>MSQPITRENFDEWMIPVYAPAPFIPVRGEGSRLWDQQGKEYIDFAGGIAVNALGHAHPELREALNEQASKFWHTGNGYTNEPVLRLAKKLIDATFADRVFFCNSGAEANEAALKLARKFAHDRYGSHKSGIVAFKNAFHGRTLFTVSAGGQPAYSQDFAPLPADIRHAAYNDINSASALIDDSTCAVIVEPIQGEGGVVPASNAFLQGLRELCNRHNALLIFDEVQTGVGRTGELYAYMHYGVTPDLLTTAKALGGGFPVGALLATEECARVMTVGTHGTTYGGNPLASAVAGKVLELINTPEMLNGVKQRHDWFVERLNTINHRYGLFSEVRGLGLLIGCVLNADYA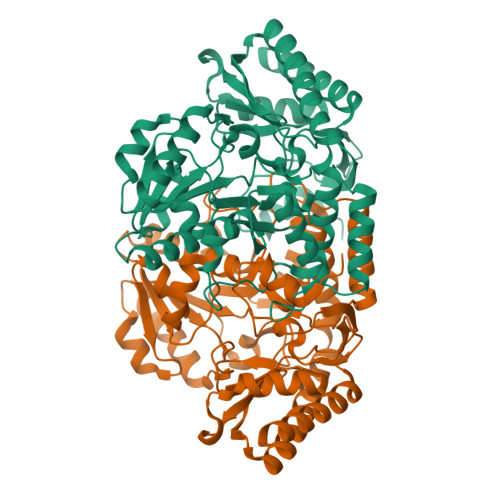GQAKQISQEAAKAGVMVLIAGGNVVRFAPALNVSEEEVTTGLDRFAAACEHFVSRGSS[2x]>[2x]MRSHILGKIELDQTRLAPDLAYLAAVPTVEEEYDEFSNGFWKHVPLWNASGDSEDRLYRDLKDAAAQPTAHVEHVPYLKEIVTTVFDGTHLQMARSRNLKNAIVIPHRDFVELDREVDRYFRTFMVLEDS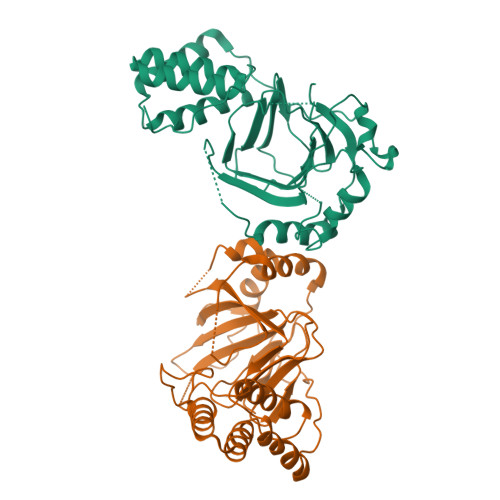PLAFHSNEDTVIHMRPGEIWFLDAATVHSAVNFSEISRQSLCVDFAFDGPFDEKEIFADATLYAPGSTPDLPERRPFTAEHRRRILSLGQVIERENFRDILFLLSKVHYKYDVHPSETYDWLIEISKQAGDEKMVVKAEQIRDFAVEARALSERFSLTSW> MHLNPAEKEKLQIFLASELALKRKARGLKLNYPEAVAIITSFIMEGARDGKTVAMLMEEGKHVLTRDDVMEGVPEMIDDIQAEATFPDGTKLVTVHNPIS;> MSNNNYIVPGEYRVAEGEIEINAGREKTTIRVSNTGDRPIQVGSHIHFVEVNKELLFDRAEGIGRRLNIPSGTAARFEPGEEMEVELTELGGNREVFGISDLTNGSVDNKELILQRAKELGYKGVE;> MKINRQQYAESYGPTVGDQVRLADTDLWIEVEKDYTTYGDEANFGGGKVLREGMGENGTYTRTENVLDLLLTNALILDYTGIYKADIGVKDGYIVGIGKGGNPDIMDGVTPNMIVGTATEVIAAEGKIVTAGGIDTHVHFINPDQVDVALANGITTLFGGGTGPAEGSKATTVTPGPWNIEKMLKSTEGLPINVGILGKGHGSSIAPIMEQIDAGAAGLKIHEDWGATPASIDRSLTVADEADVQVAIHSDTLNEAGFLEDTLRAINGRVIHSFHVEGAGGGHAPDIMAMAGHPNVLPSSTNPTRPFTVNTIDEHLDMLMVCHHLKQNIPEDVAFADSRIRPETIAAEDILHDLGIISMMSTDALAMGRAGEMVLRTWQTADKMKKQRGPLAEEKNGSDNFRAKRYVSKYTINPAIAQGIAHEVGSIEEGKFADLVLWEPKFFGV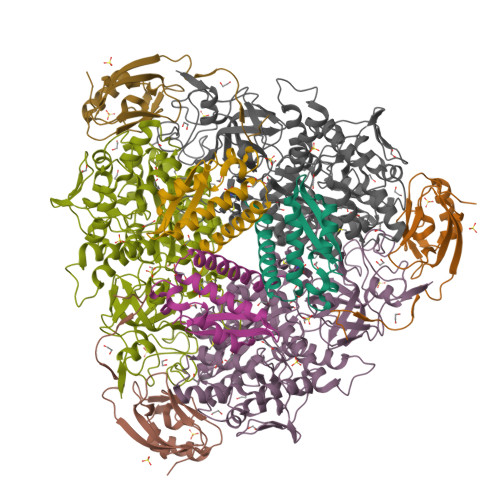KADRVIKGGIIAYAQIGDPSASIPTPQPVMGRRMYGTVGDLIHDTNITFMSKSSIQQGVPAKLGLKRRIGTVKNCRNIGKKDMKWNDVTTDIDINPETYEVKVDGEVLTCEPVKELPMAQRYFLF>[2x]MVKLAEFSRTATFAWSHDKIPLLVSGTVSGTVDANFSTDSSLELWSLLAADSEKPIASLQVDSKFNDLDWSHNNKIIAGALDNGSLELYSTNEANNAINSMARFSNHSSSVKTVKFNAKQDNVLASGGNNGEIFIWDMNKCTESPSNYTPLTPGQSMSSVDEVISLAWNQSLAHVFASAGSSNFASIWDLKAKKEVIHLSYTSPNSGIKQQLSVVEWHPKNSTRVATATGSDNDPSILIWDLRNANTPLQTLNQGHQKGILSLDWCHQDEHLLLSSGRDNTVLLWNPESAEQLSQFPARGNWCFKTKFAPEAPDLFACASFDNKIEVQTLQNLTNTLDEQETETKQQESETDFWNNVSREESKEKPSVFHLQAPTWYGEPSPAAHWAFGGKLVQITPDGKGVSITNPKISGLESNTTLSEALKTKDFKPLINQRLVKVIDDVNEEDWNLLEKLSMDGTEEFLKEALAFDNDESDAQDDANNEKEDDGEEFFQQIETNFQPEGDFSLSGNIEQTISKNLVSGNIKSAVKNSLENDLLMEAMVIALDSNNERLKESVKNAYFAKYGSKSSLSRILYSISKREVDDLVENLDVSQWKFISKAIQNLYPNDIAQRNEMLIKLGDRLKENGHRQDSLTLYLAAGSLDKVASIWLSEFPDLEDKLKKDNKTIYEAHSECLTEFIERFTVFSNFINGSSTINNEQLIAKFLEFINLTTSTGNFELATEFLNSLPSDNEEVKTEKARVLIASGKSLPAQNPATATTSKAKYTNAKTNKNVPVLPTPGMPSTTSIPSMQAPFYGMTPGASANALPPKPYVPATTTSAPVHTEGKYAPPSQPSMASPFVNKTNSSTRLNSFAPPPNPYATATVPATNVSTTSIPQNTFAPIQPGMPIMGDYNAQSSSIPSQPPINAVSGQTPHLNRKANDGWNDLPLKVKEKPSRAKAVSVAPPNILSTPTPLNGIPANAAST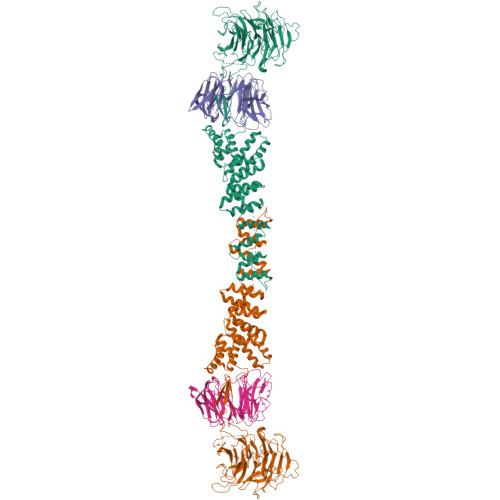MPPPPLSRAPSSVSMVSPPPLHKNSRVPSLVATSESPRASISNPYAPPQSSQQFPIGTISTANQTSNTAQVASSNPYAPPPQQRVATPLSGGVPPAPLPKASNPYAPTATTQPNGSSYPPTGPYTNNHTMTSPPPVFNKPPTGPPPISMKKRSNKLASIEQNPSQGATYPPTLSSSASPLQPSQPPTLASQVNTSAENVSHEIPADQQPIVDFLKEELARVTPLTPKEYSKQLKDCDKRLKILFYHLEKQDLLTQPTIDCLHDLVALMKEKKYKEAMVIHANIATNHAQEGGNWLTGVKRLIGIAEATLN;> VVIANAHNELIHDAVLDYYGKRLATCSSDKTIKIFEVEGETHKLIDTLTGHEGPVWRVDWAHPKFGTILASCSYDGKVLIWKEENGRWSQIAVHAVHSASVNSVQWAPHEYGPLLLVASSDGKVSVVEFKENGTTSPIIIDAHAIGVNSASWAPATIEEDGEHNGTKESRKFVTGGADNLVKIWKYNSDAQTYVLESTLEGHSDWVRDVAWSPTVLLRSYLASVSQDRTCIIWTQDNEQGPWKKTLLKEEKFPDVLWRASWSLSGNVLALSGGDNKVTLWKENLEGKWEPA;> VVIANAHNEMIHDAVMDYYGKRMATCSSDKTIKIFEVEGETHKLIDTLTGHEGPVWRVDWAHPKFGTILASCSYDGKVMIWKEENGRWSQIAVHAVHSASVNSVQWAPHEYGPMLLVASSDGKVSVVEFKENGTTSPIIIDAHAIGVNSASWAPATIEEDGEHNGTKESRKFVTGGADNLVKIWKYNSDAQTYVLESTLEGHSDWVRDVAWSPTVLLRSYMASVSQDRTCIIWTQDNEQGPWKKTLLKEEKFPDVLWRASWSLSGNVLALSGGDNKVTLWKENLEGKWEPA> MGSSHHHHHHSSGRENLYFQGHMNDFSLELPVRTNKPRETGQSILIDNGYPLQFFKDAIAGASDYIDFVKFGWGTSLLTKDLEEKISTLKEHDITFFFGGTLFEKYVSQKKVNEFHRYCTYFGCEY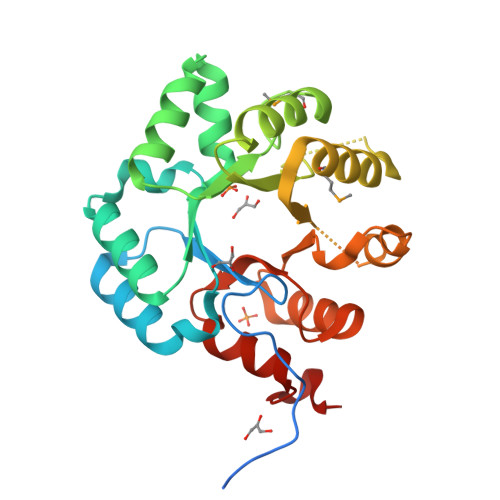IEISNGTLPMTNKEKAAYIADFSDEFLVLSEVGSKDAELASRQSSEEWLEYIVEDMEAGAEKVITEARESGTGGICSSSGDVRFQIVDDIISSDIDINRLIFEAPNKTLQQGFIQKIGPNVNLANIPFHDAIALETLRLGLRSDTFFLGS> MKRADDFQQRRAHLANLSDEELQTRFWEM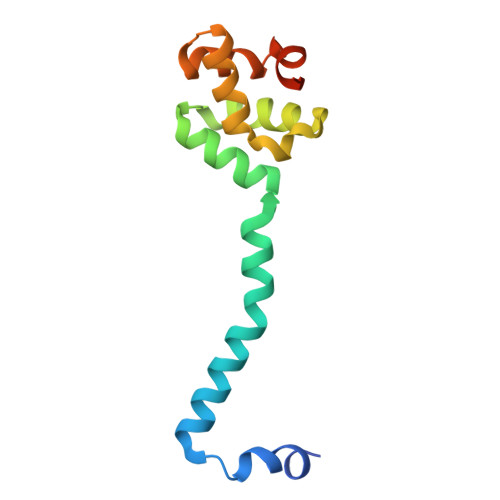AEKIVDPLLDLGKKNTTPSIERSVLLRMGFSSLEAKAIVDKTMDRGLMGKGAGHIVYKIAKEKNISVREAGLALSEGKYWDDAIQIFKGGVK>VTPPPEKFNFAEHLLQTNRVRPDKTAFVDDISSLSFAQLEAQTRQLAAALRAIGVKREERVLLLMLDGTDWPVAFLGAIYAGIVPVAVNTLLTADDYAYMLEHSRAQAVLVSGALHPVLKAALTKSD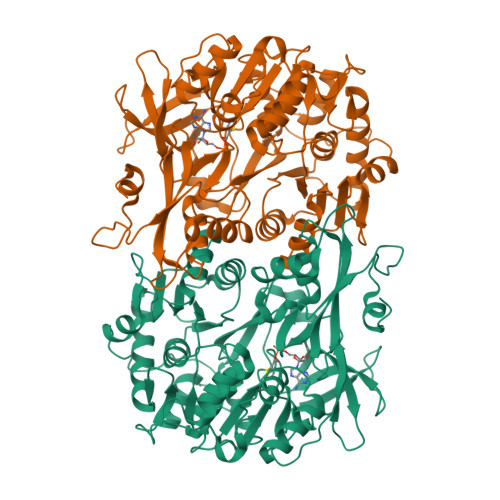HEVQRVIVSRPAAPLEPGEVDFAEFVGAHAPLEKPAATQADDPAFWLYSSGSTGRPKGVVHTHANPYWTSELYGRNTLHLREDDVCFSAAKLFFAYGLGNALTFPMTVGATTLLMGERPTPDAVFKRWLGGVGGVKPTVFYGAPTGYAGMLAAPNLPSRDQVALRLASSAGEALPAEIGQRFQRHFGLDIVDGIGSTEMLAAFLSNLPDRVRYGTTGWPVPGYQIELRGDGGGPVADGEPGDLYIHGPSSATMYWGNRAKSRDTFQGGWTKSGDKYVRNDDGSYTYAGRTDDMLKVSGIYVSPFEIEATLVQHPGVLEAAVVGVADEHGLTKPKAYVVPRPGQTLSETELKTFIKDRLAPYKYPRSTVFVAELPKTATGKIQRFKLREGVL[2x]>AAHGMEEELVVISKSIVNPRSLKKPTSVKKIQLTPWDLSRLRFGYLQRGLLFHKIEVKQLQASLSVALDRFYPLAGRLVKLKNDDDTVSFFISCDGSGVEFVHAVAKNIELSDVLELSGSVPGFFASFFPATGIKNYHGVSRSLLMVQVTEMKDGVFIGFGYNSTVADATSIWKFINAWSEICSKDSSGSQTFQRRLHLKGWFFDEIDYPIHIPDPETKPTSYVTTPTNLQEKMFHVTKENVLKLDAKANDEADQKISSIQAVLAYIWRSMVKHSGMSREEETHCRLPINMRQRLNPPLEEECFGNVSQTGIATVTVGELLDHGLGWAAMQINNMELSQTDEKAKAFAENWVKNIKIPVSVGS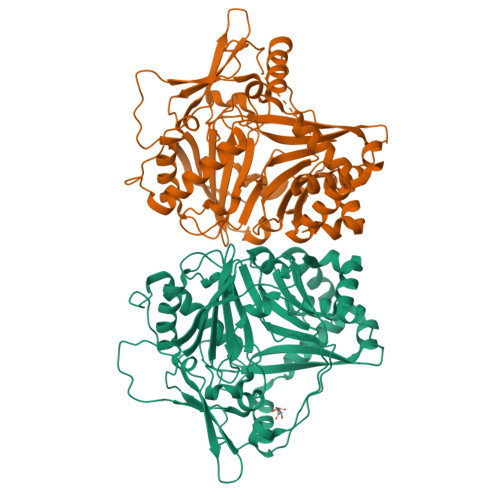KDLVVTNSHRFDVYCNDFGWGKPIAARAGPPYLNGRLVVFKGIGEASLDFQACLLPQVVEKLVKDAEFNEYVSIV[2x]>MTQATPSFETLRYAVADGVATITLHRPDQLNAFTAQMMHELIAAFDATDADDNVRAVIVTGSGRAFCAGADLSGGSSTFDFEKRYGASPDSAHRDGGGRVSLRIFRSLKPVIAAVNGAAVGVGVTMQLPMDIRLASTDAKFGFVFARRGITPEAASSWFLSRVVGISTALEWCYTGRVFSAQEAHERGLVRSLHAPEDLLPAAQAIAREIAANAAPVSVAISRQLIWRMAGASHPMEAHKLDSRAIQSRGRSADVKEGVSAFL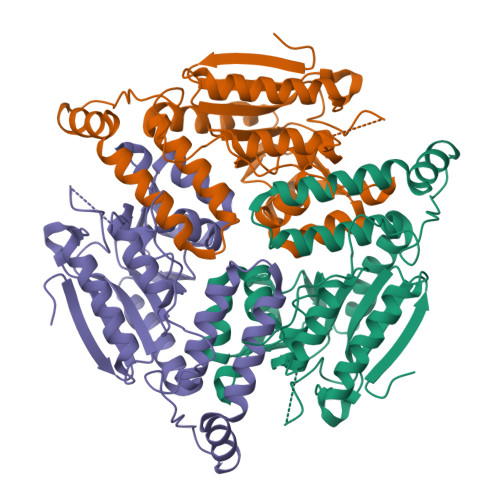EKRPAAFPETVSHDMPDFFDWTSEPPFILEHHHHHH[2x]>[6x]MAQGTLYIVSAPSGAGKSSLIQ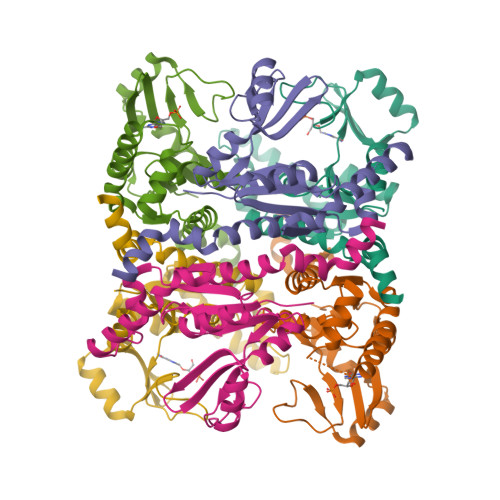ALLKTQPLYDTQVSVSHTTRQPRPGEVHGEHYFFVNHDEFKEMISRDAFLEHAEVFGNYYGTSREAIEQVLATGVDVFLDIDWQGAQQIRQKMPHARSIFILPPSKIELDRRLRGRGQDSEEVIAKRMAQAVAEMSHYAEYDYLIVNDDFDTALTDLKTIIRAERLRMSRQKQRHDALISKLLAD> TECDFSPMFKGVAPQVYNFKRLVFSNCNYNLTKLLSLFAVDEFSCNGISPDAIARGCYSTLTVDYFAYPLSMKSYIRPGSAGNIPLYNYKQSFAHPTCRVLA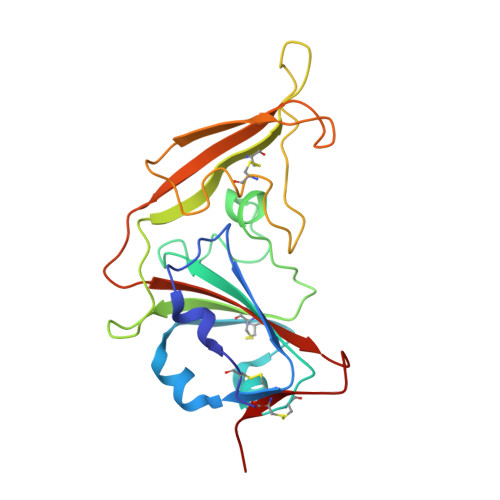SVPPNVTITKPEAYGYISKCSRLTGDYQHIETPLYINPGEYSICRDFAPLGFSEDGQVFKRTLTQFEGGGLLIGVGTRVPMTANLEMGFVISVQYGAGTDSVCPMLD2-cyclohexyl-N-(5-sulfamoyl-1,3,4-thiadiazol-2-yl)acetamide | C10 H16 N4 O3 S2 | 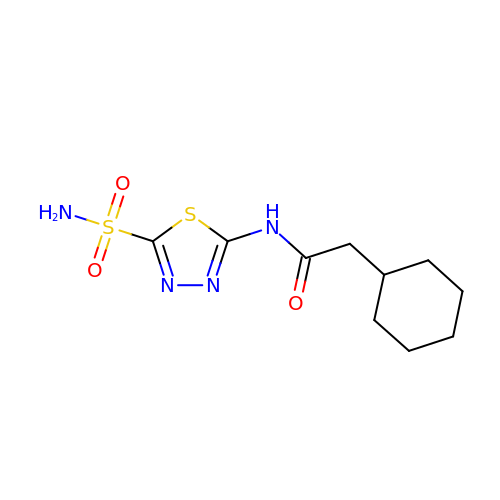JUBREXAVHBVMRO-UHFFFAOYSA-N>[2x]MIKEIYLAGGSFWGVEGYFRQIPGVKETDTGYANGKNDSANYKGLHQSDHAETVKIVYDS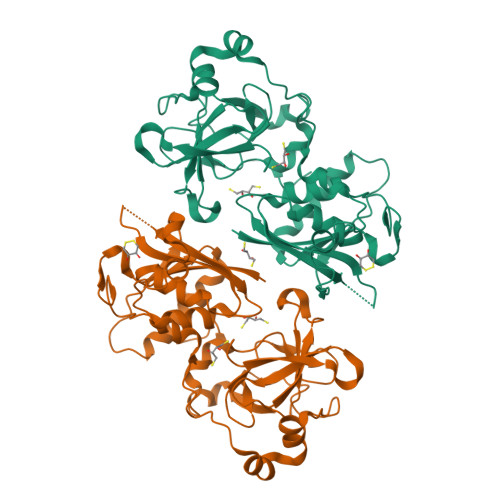SVVSLQELLAHYFRIIDPTSLNKQGNDAGRQYRTGIYYVDDSMIKEINSFVKFMQKKYSRPIVVEVEKLKHFILAEDYHQDYLQKNPGGYCHIDLTLALKPLYDESKFKVPSKEELKKSLKPIQFSVTQEKATERPFTSEYDKFDAEGIYVDITTGKPLFSSLNKYDAGCGWPSFTKAITTQALQYLEDKSLGMNRTEVVSKTGGAHLGHVFDDGPADAGGLRYSINGAALRFIPYDKMEKEGYGDYLPYVKPTGNFLEHHHHHH> LKTK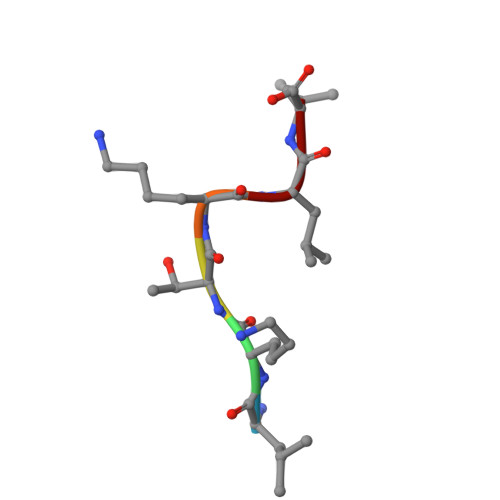LL7-{[(2S)-2-butyl-6,7-dichloro-2-cyclopentyl-1-oxo-2,3-dihydro-1H-inden-5-yl]oxy}heptanoic 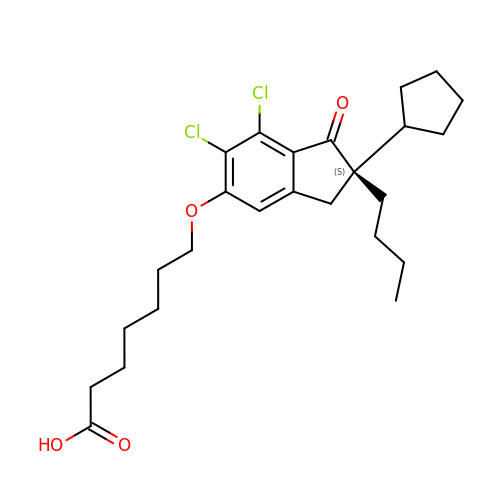acid | C25 H34 Cl2 O4 | FIDRMVPJOHBYQH-VWLOTQADSA-N> AF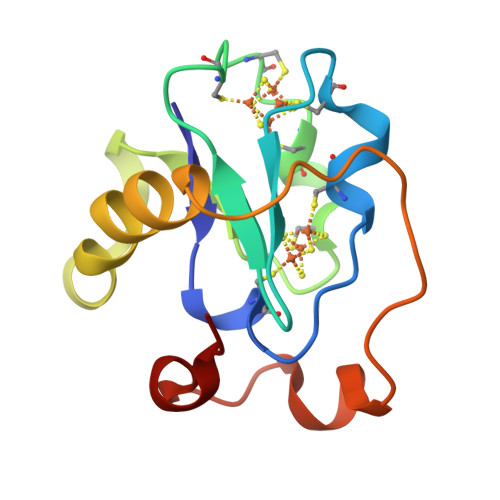VVTDNCIKCKYTDCVEVCPVDAFYEGPNFLVIHPDECIDCALCEPECPAQAIFSEDEVPEDMQEFIQLNAELAEVWPNITEKKDPLPDAEDWDGVKGKLQHLER> WKEIK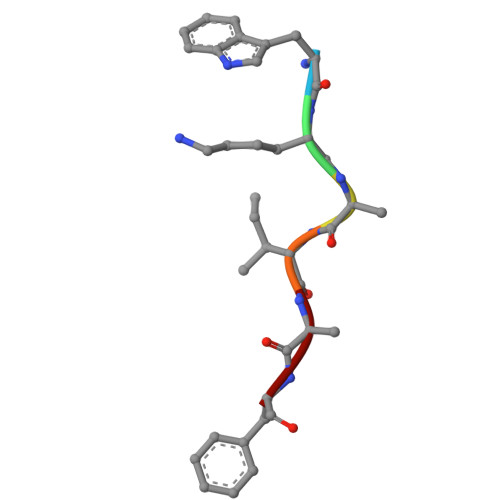F>[2x]GHMFGSINLASSLSVDAPGLQNQIDELSSFSDAPSPSVTRVLYTDKDVSARRYVKNLMALAGLTVREDAVGNIFGKWDGLEPNLPAVATGSHIDAIPYSGKYDGVVGVLGAIEAINVLKRSGFKPKRSLE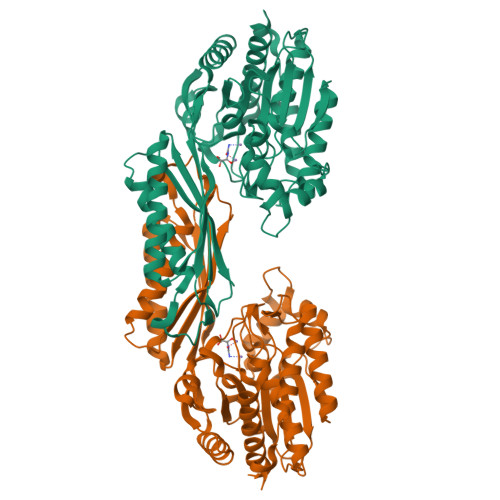IILFTSAEPTRFGISCLGSRLLAGSKELAEALKTTVVDGQNVSFIEAARSAGYAEDKDDDLSSVFLKKGSYFAFLELHIEQGPILEDEGLDIGVVTAIAAPASLKVEFEGNGGHAGAVLMPYRNDAGLAAAELALAVEKHVLESESIDTVGTVGILELHPGAINSIPSKSHLEIDTRDIDEARRNTVIKKIQESANTIAKKRKVKLSEFKIVNQDPPALSDKLVIKKMAEAATELNLSHKMMISRAYHDSLFMARISPMGMIFIPCYKGYSHKPEEYSSPEDMANGVKVLSLTLAKLSLD> MATRLDRLVTILETGSTRLIRDTAVNQLADWQKQHPEELFNLLSRVVPYLRHKDWETRTTAAKAIGKIIENAPLYDPNAGQDEAAPEPTNGSFEVKKEEEKDVLEQDNFFRLESLDVATIVKYGRPLLRGGPVDYNLAALDPQKRLAHLKKTLNGRLGLLGRVFEDEEMPVEQIASPITPNDAAGANGVGRQDGASNDNQSQAIDESKMSARQLNVLKRKRKREAQKAAQGKSGFGDLSLRRSTTAGSDAFGEDTPMPDADSKKNKLAEYFSLDRPENTEEDTKIVSEFKGPVLPIKSEIEADDSLEGAEWPFERLCEFLKVDLFDPQWETRHGAAMGLREVIRVHGAGAGRRRGKTRKENNDLNRQWLDDLAYRLLCVLMLDKFTDYSSDTSVAPIRETVGQTLGAVLRHISVESVHAIYRLLYCMVTQEDLPSEQNMWAVCHGGMVGLRYVVAVRKDLLLQDGDMIDGVVRCVMQGLGDIDDDVRSVSAATLIPMAKEFVMMRRSALDSLINIVWESLSNLGDDLSASTGKIMDLLATLCSFPEVLEAMKVSASQDEERSFTLLVPRLYPFLRHTITSVRLAVLKALMTFANLGGETSQGWLNGRILRLIFQNIIVERDQDTLNMSLELWTTLVRRLAARDPAILADEFEAHAEPMMQLALHPIGVPRHPIPMNPALFQKPSGGTYSLPGASQTNSRRSSPPEGERATKRRRKSTKAEDVAPSTHTHDVDGHMIQGEVDLVGVDVLIRSRISAAKAMGLIMSFIPTPRLASYDTAVLQALSSPYASTQLAAAMVIDEYAKNCSTPEVASRFIEPLQKIIDLERP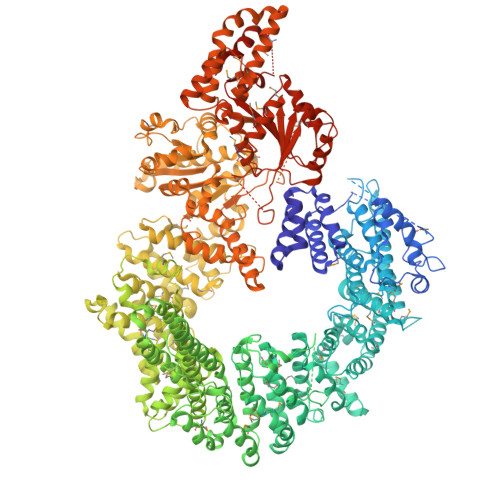SHYRDLVTYVQRVRSASQQLINLFRDHGKVSQGKLPTLAVVVQGEPEAGPGAFSIANAEKVVNEDFERLKRLMAPGQRLIALPQLNEAREQTVEVIEEAKAAKEARDARIKAAAACALVAMKVLPKKPSPLIKAIMDSIKTEENQELQSRSAATIARLVQLFTESGRRGPAEKVVANLVKFSCVEVAETPEFPIHAHKTNVILSMQKEEDRVDHPDAVKYAREAKAARITRRGAKEALEILSKNFGAELLERVPTLRTFMEEPLVRAFSGDLPPEARDPENAFGQEIVDAMSVIRTMTPTLHPALHPFVMQQVPLVIKALRSDLSVFRYMAAKCMATICSVITVDGMTALVEKVLPSINNPLDLSFRQGAIEVIYHLIAVMGDAILPYVIFLIVPVLGRMSDSDNQIRLIATTSFATLVKLVPLEAGIPDPPGLSEELLKGRDRERTFIAQLLDPKKIEPFKIPVAIKAELRSYQQEGVNWLAFLNKYHLHGILCDDMGLGKTLQTICIVASDHHQRAEEFARTGAPEVRKLPSLIICPPTLSGHWQQEIKTYAPFLTVTAYVGSPAERRAMKDSLDKTDIVITSYDVCRNDIDVIEKYNWNYCVLDQGHLIKNPKAKITLAVKRLTSNHRLILTGTPIQNNVLELWSLFDFLMPGFLGAEKVFLDRFAKPIANSRYSKASSKEQEAGALAIEALHKQVLPFLLRRLKEEVLNDLPPKILQNYYCDLSDLQRKLFEDFTKREGKKITETAGRDDKEAKQHIFQALQYMRKLCNSPALVMKPGHKAYEDTQKYLAKHGTTLEDPIHAPKLGALRDLLVDCGIGVEGQESSDPLYTPIKPHRALIFCQMKEMLDMVQNTVLKQMLPSVSYLRLDGSVEANKRQDIVNKFNSDPSYDVLLLTTSVGGLGLNLTGADTVIFVEHDWNPQKDLQAMDRAHRIGQKKVVNVYRIITRGTLEEKILSLQRFKIDVASTVVNQQNAGLATMDTDQILDLFNLGESGPSLITDNKESIELEVLFQGPHHHHHHHH>[4x]MSAANADFELFRVFLEKTCGIVLG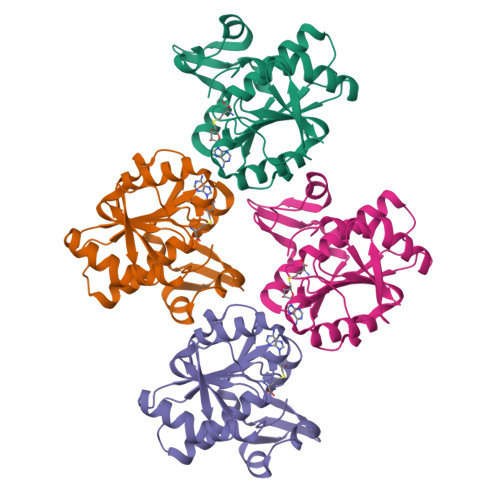SNKQYLVSSRLNKLMEQQGIKSLGELVQRIQTQRGGLREMVVDAMTTNETLWFRDTYPFEVLKQRVLPELIKANGGQRLRIWSAACSSGQEPYSLSMAIDEFEKTNLGQLKAGVQIVATDLSGSMLTAAKAGEYDTLAMGRGLSPERLQRYFDAKGPGRWAVKPAIRSRVEFRALNLLDSYASLGKFDMVFCRNVLIYFSAEVKRDILLRIHGTLKPGGYLFLGASEALNNLPDHYQMVQCSPGIIYRAKLEHHHHHH>[66x]SFSQAVSGLNAAATNLDVIGNNIANSATYGFKSGTASFADMFAGSKVGLGVKVAGITQDFTDGTTTNTGRGLDVAISQNGFFRLVDSNGSVFYSRNGQFKLDENRNLVNMQGMQLTGYPATGTPPTIQQGANPAPITIPNTLMAAKSTTTASMQINLNSTDPVPSKTPFSVSDADSYNKKGTVTVYDSQGNAHDMNVYFVKTKDNEWAVYTHDSS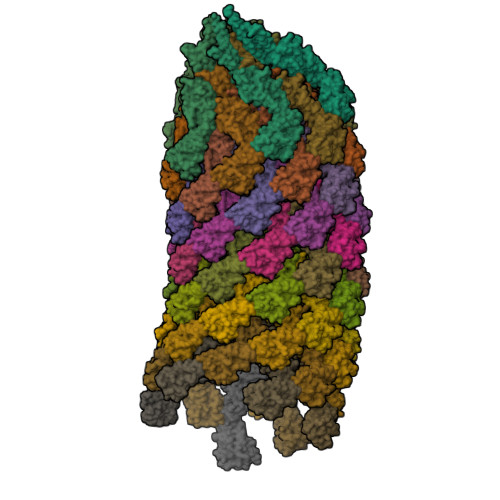DPAATAPTTASTTLKFNENGILESGGTVNITTGTINGATAATFSLSFLNSMQQNTGANNIVATNQNGYKPGDLVSYQINNDGTVVGNYSNEQEQVLGQIVLANFANNEGLASQGDNVWAATQASGVALLGTAGSGNFGKLTNGALEASNVDLSKELVNMIVAQRNYQSNAQTIKTQDQILNTLVNLR>MEAKAIARYVRISPRKVRLVV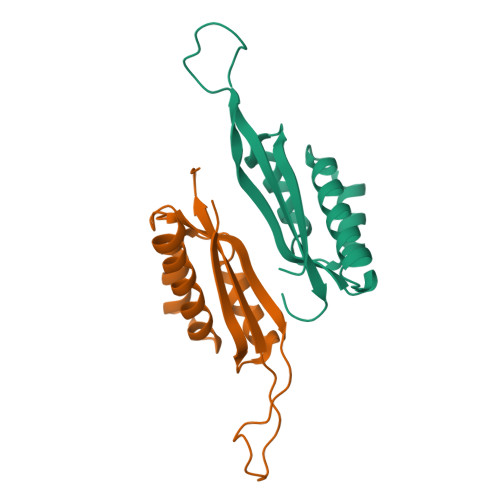DLIRGKSLEEARNILRYTNKRGAYFVAKVLESAAANAVNNHDALEDRLYVKAAYVDEGPAVLPRARGRADIIKKRTSHITVILGEKHGK[2x]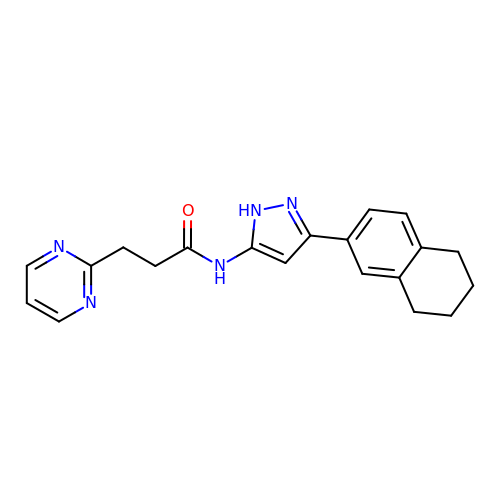3-(pyrimidin-2-yl)-N-[3-(5,6,7,8-tetrahydronaphthalen-2-yl)-1H-pyrazol-5-yl]propanamide | C20 H21 N5 O | YOAVNWPBYNWYQZ-UHFFFAOYSA-N>[2x]MADEIAKAQVARPGGDTIFGKIIRKEIPAKIIFEDDRCLAFHDISPQAPTHFLVIPKKHISQISVAEDDDESLLGHLMIVGKKCAADLGLNKGYRMVVNEGSDGGQSVYHVHLHVLGGRQMHWPPG

Histidine triad nucleotide-binding proteins (HINTs) exhibit hydrolytic activity toward nucleoside phosphoramidates, such as tryptamine adenosine phosphoramidate (TrpA). While the biologically relevant substrates of HINT1 have not been clearly elucidated, the protein has been implicated in opioid receptor signaling, − regulation of the melanoma-associated transcription factor MITF, , and DNA damage repair. These functions position HINT1 as a potential pharmacological target for treating conditions such as opioid resistance or melanoma.

Our initial screening library included three additional hydroxamic acids with 4-(heteroaryl)-phenyl motifs: KV-24, KV-30, and KV-50, which were proteomically characterized alongside the SW-100 analogs. While these compounds initially appeared to demonstrate excellent selectivity for MBLAC2 over HDAC6, we unexpectedly observed dose-dependent competition of several other proteins in chemoproteomic competition experiments. These compounds also bound to HINT1 and NME4, and, with lower affinity, HINT2 and a protein ambiguously identified as NME1 or NME2. The only reported HINT1-targeting pharmacophores are nucleoside-based nonhydrolyzable substrate analogs, such as the carbamate TrpGC. ,, We evaluated the inhibitory potential of KV-24 and KV-30 in enzyme activity assays using recombinant HINT1. Both compounds effectively inhibited HINT1 activity, with half-maximal inhibitory concentrations (IC50) of 12.3 μM for KV-24 and 12.6 μM for KV-30, which are comparable to the state-of-the-art HINT1 inhibitor TrpGC (IC50 = 9.1 μM). The structures revealed that the aromatic ring systems of KV-24 and KV-30 are buried in a hydrophobic cleft typically occupied by the base of the substrate nucleoside. This finding supports a competitive inhibition mode of action. Additionally, casein kinase 2 family members exhibited reduced binding at two-digit μM concentrations of KV-24. Interestingly, KV-24 showed dose-dependent binding to calcium/calmodulin-dependent 3′,5′-cyclic nucleotide phosphodiesterase 1C (PDE1C), with an affinity of approximately 2 μM. PDE1C is a cAMP/cGMP nucleotide-binding protein that features two divalent metal cation cofactors. The hydroxamic acid moiety of KV-24 might chelate these metal cofactors, supporting the hypothesis that KV-24 binds the active site of PDE1C. Thus, KV-24 and KV-30 should be regarded only as preliminary scaffolds for developing more selective inhibitors.1,2,5-trimethyl-1H-pyrrole-3-carboxylic 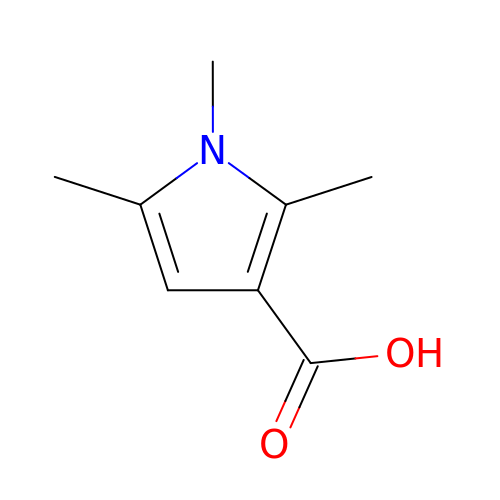acid | C8 H11 N O2 | JTEBLTWGSAXWEE-UHFFFAOYSA-N> MASEAIKGAVVGIDLGTTNSCVAVMEGKQAKVLENAEGARTTPSVVAFTADGERLVGMPAKRQAVTNPNNTFYATKRLIGWRYDDPEVQKDIKNVPFKIVRASNGDAWVEAHGKLYSPSQIGAFVLMKMKETAENYLGHTAKNAVITVPAYFNDSQRQATKDAGQISGLNVLRVINEP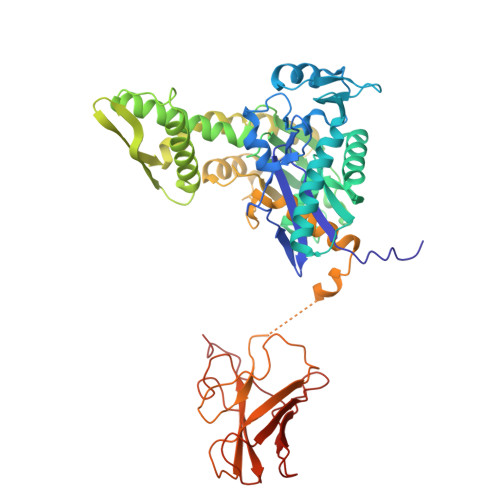TAAALAYGLDKSEDKVIAVYDLGGGTFDISILEIQKGVFEVKSTNGDTFLGGEDFDQALLRHIVKEFKRETGVDLTKDNMALQRVREAAEKAKCELSSSVQTDINLPYLTMDSSGPKHLNMKLTRAQFEGIVTDLIRRTIAPCQKAMQDAEVSKSDIGEVILVGGMTRMPKVQQTVQDLFGRAPSKAVNPDEAVAIGAAIQGGVLAGDVTDVLLLDVTPLSLGIETLGGVFTKLINRNTTIPTKKSQVFSTAADGQTQVEIKVCQGEREMAGDNKLLGQFTLIGIPPAPRGVPQIEVTFDIDANGIVHVSAKDKGTGREQQIVIQSSGGLSKDDIE>[3x]MASNFTQFVLVDNGGTGDVTVAPSNFANGVAEWISSNSRSQAYKVTCSVRQSSAQNRKYTIKVEVPKVATQTVGGVELPVAAWRSYLNME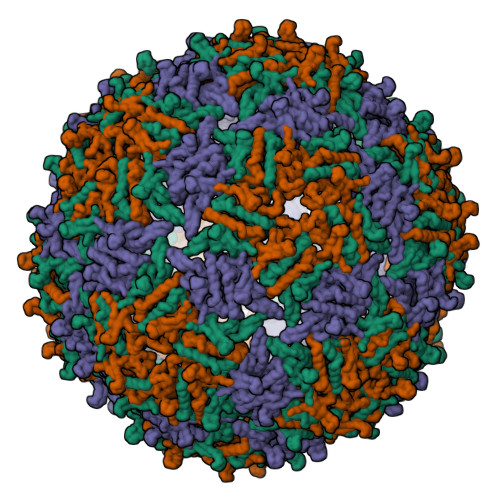LTIPIFATNSDCELIVKAMQGLLKDGNPIPSAIAANSGIY> SLMERLGGGGFSARIFVGLNVGDKPTYTIEDVVKDTIAIRKRQGILPDASFVAQRGVYTEQRSGQLVTENSVQIIIIDLEGLSKEDFTGKVQALGKELREDFKQESVIVEIQERGIVQDVYSITAEWYEEGPMRPLRVDLQPSLI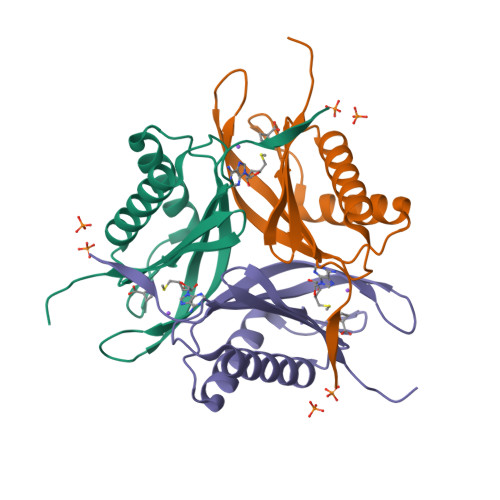S> GSDTSGILLASITGAGSAFQAYAGCYLTAFRNDPRTLTLRMDKTRGERISNVLVILSGGAL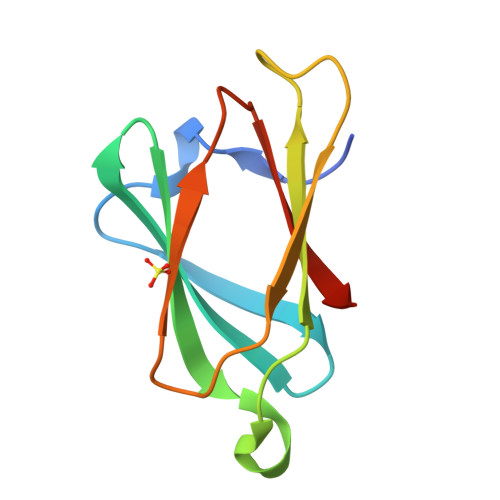SHAVEEVVQIAPGAVRNLATLGASTVQFLHNFRS> GDCTGKLRGNVAANKETTFQGLTIA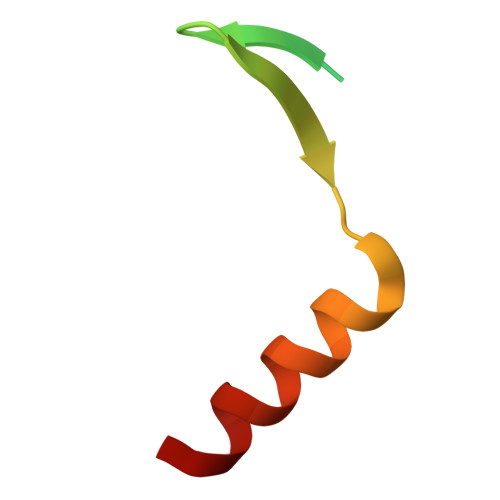SGARESEKVFAQTVLSHV> MHHHHHHMFGIGTKDLGIDLGTANTLVYVKGKGIVLREPSVVAIQRDTKQIVAVGNEAKNMIGRTPGNIVALRPMKDGVIADYETTATMMKYYIRKAIKTKGLFAGKPYVMVCVPYGITAVEERAVIDATRQAGARDAYTIEEPFAAAIGANLPVWEPTGSMVVDIGGGTTEVAVISLGGIVTSQSIRIAGDEMDEAIIQYIRKSYNLMIGERTAEAIKMEIGSAGNPEGIGNMEIRGRDLLTGLPKTIEISAEEVAEALRDTVYAIVESVKNTLEKTPPELAADIMDRGIVLTGGGALLRNLDKVISQETDMPVIVAENPLDCVAIGTGKALDHIDLFKNKARDHR

In vivo, MreB proteins form discrete, nanometer-long, membrane-associated polymeric assemblies along the cell cylinder that move processively around the rod circumference together with proteins of the cell wall (CW) elongation machinery, forming the so-called Rod complex. The current model is that self-aligned MreB filaments restrict the diffusion of CW biosynthetic proteins in the membrane and orient their motion to insert new peptidoglycan strands in radial hoops perpendicular to the long axis of the cell, promoting the cylindrical expansion of rod-shaped cells. We successfully purified a soluble form of MreB from the Gram-positive thermophilic Geobacillus stearothermophilus (MreBGs) and elucidated its crystal structure, confirming the classical actin/MreB fold and the presence of the small hydrophobic loop shown to mediate membrane binding in MreBTm and MreB5Sc. We also show that the interaction with lipids is mediated by electrostatic interactions and by two spatially close hydrophobic motifs in the MreBGs monomers that comprise the small hydrophobic loop and the N-terminal end.

The electron density map clearly revealed the presence of three phosphates, demonstrating that the ATP had not been hydrolyzed into ADP. This is probably due to the absence of a Mg2+ ion in the catalytic site. No residual electron density peak could be interpreted as a Mg2+ ion with appropriate coordination. As a consequence, the binding mode of the nucleotide is distinct from other MreB structures, with the γ-phosphate located in the Mg2+ binding site. The structure of the ATP-bound form of MreBGs is highly similar to the apo form, with a rmsd of 1.41 Å over 313 aligned Cα atoms. However, ATP binding induced a small closure of the nucleotide-binding pocket, and loop β6-α2, which was disordered in the apo structure, is fully visible in the electron density map. The hydrophobic loop α2-β7 and the N-terminus also display an alternative conformation. Despite multiple co-crystallization trials, in the ATP-bound state the crystal packing only revealed monomers and never straight protofilaments as in the apo structure. Comparison of the crystal structures of apo and ATP-bound MreBGs shows that only minor conformational changes occur upon nucleotide-binding, in agreement with what was observed when comparing crystal structures of MreBCc and MreB5Sc in different nucleotide-bound states.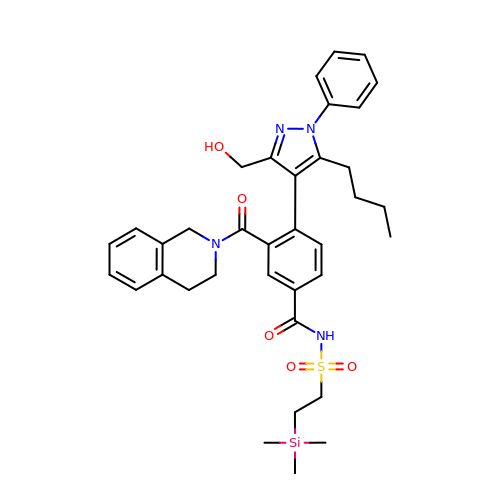4-[5-butyl-3-(hydroxymethyl)-1-phenyl-1H-pyrazol-4-yl]-3-(3,4-dihydroisoquinolin-2(1H)-ylcarbonyl)-N-{[2-(trimethylsilyl)ethyl]sulfonyl}benzamide | C36 H44 N4 O5 S Si | KDMMHDWLRNJPDK-UHFFFAOYSA-N>[3x]SIDVKYIGVKSAYVSYDVQKRTIYLNITNTLNITNNNYYSVEVENITAQVQFSKTVIGKARLNNITIIGPLDMKQIDYTVPTVIAEEMSYMYDFCTL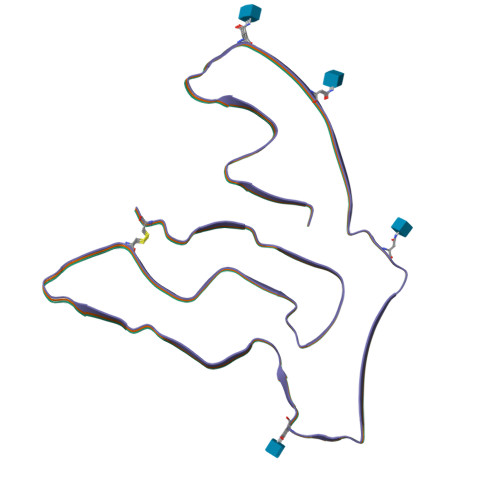ISIKVHNIVLMMQVTVTTTYFGHSEQISQERYQYVDCG> GQNHHEVVKFMDVYQRSYCHPIETLVDIFQEYPDEIEYIFKPSCVPLMRCGGCCNDEGLECVPTEESNITMQIMRIKPHQGQHIGEMSFLQHNKCECRPKKD;> CA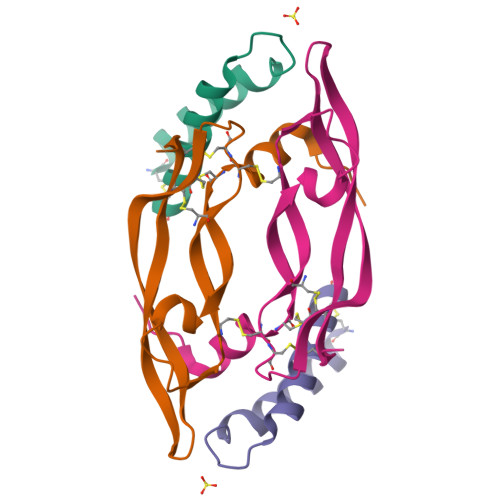AELAALEAELAALEGHVEEADFPWGKLNNLIEKLWQLKQACX>[2x]NGEAICSALPTIPYHKLADLRYLSRGASGTVSSARHADWRVQVAVKHLHIHTPLLDSERKD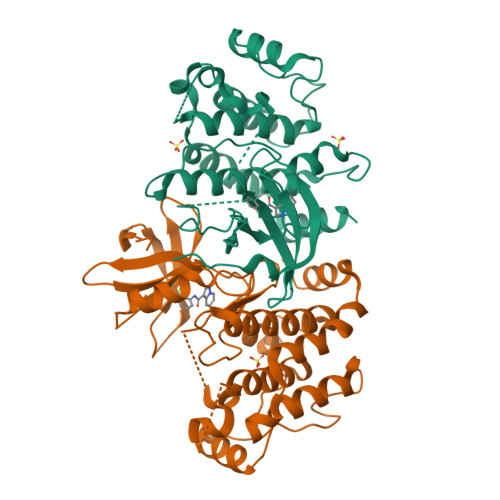VLREAEILHKARFSYILPILGICNEPEFLGIVTEYMPNGSLNELLHRKTEYPDVAWPLRFRILHEIALGVNYLHNMTPPLLHHDLKTQNILLDNEFHVKIADFGLSKWRMMSLSQSRSSKSAPEGGTIIYMPPENYEPGQKSRASIKHDIYSYAVITWEVLSRKQPFEDVTNPLQIMYSVSQGHRPVINEESLPYDIPHRARMISLIESGWAQNPDERPSFLKCLIELEPVLRTFEEITFLEAVIQLKK> X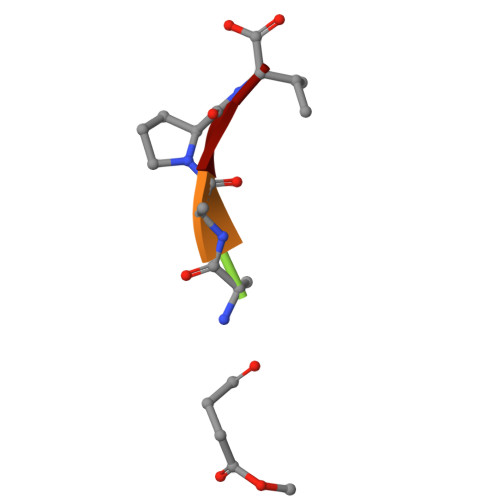AAPV tert-butyl (3R)-3-({5-[(Z)-(5-{[(1R)-1-(4-fluorophenyl)ethyl]carbamoyl}-2-oxo-1,2-dihydro-3H-indol-3-ylidene)methyl]-2,4-dimethyl-1H-pyrrol-3-yl}carbamoyl)piperazine-1-carboxylate 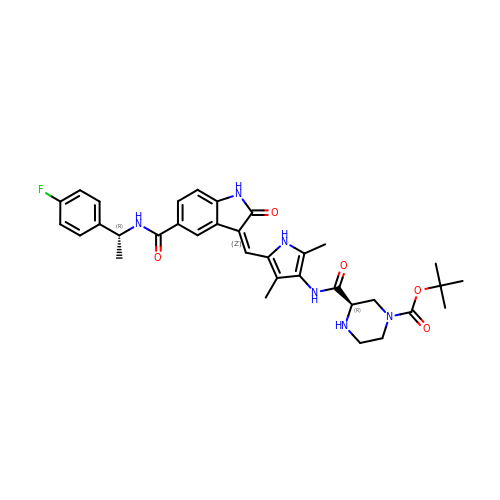| C34 H39 F N6 O5 | BISREQDPCIZZMG-WHLCRQNOSA-N>[5x]QANLMRLKSDLFNRSPMYPGPTKDDPLTVTLGFTLQDIVKVDSSTNEVDLVYYERQRWKLNSLMWDPNEYGNITDFRTSAADIWTPDITAYESTRPVQVLSPQIAVVTHDG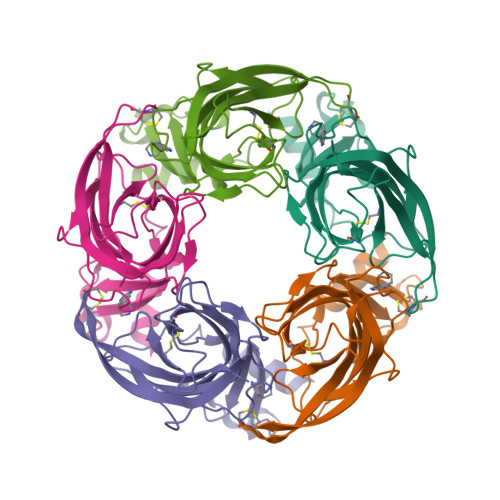SVMFIPAQRLSFMCDPTGVDSEEGVTCALTFGSWVYSGFEIDLKTDTDQVDLSSYYASSKYEILSATQTRQVQHYSCCPEPYIDVNLVVKFRERRAGNGFF> FEKCGKRVDRLDQRRSKLR;> VVGGHPGNSPWTVSLRNRQGQHFCGGSLVKEQWILTARQCFSSCHMPLTGYEVWLGTLFQNPQHGEPSLQRVPVAKMVCGPSGSQLVLLKLERSVTLNQRVALICLPPEWYVVPPGTKCEIAGWGETKGTGNDTVLNVALLNVISNQECNIKHRGRVRESEMCTEGLLAPVGACEGDYG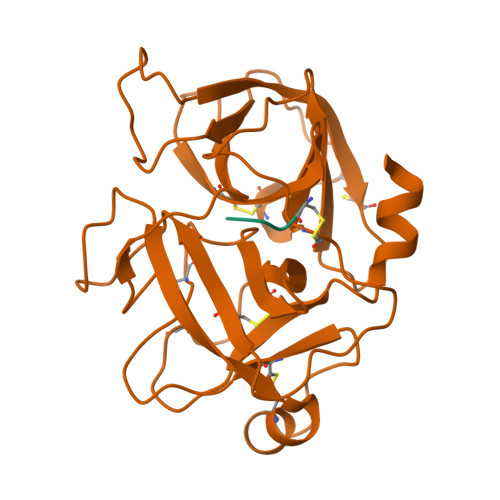GPLACFTHNSWVLEGIIIPNRVCARSRWPAVFTRVSVFVDWIHKVMRLGHHHHHH> SSN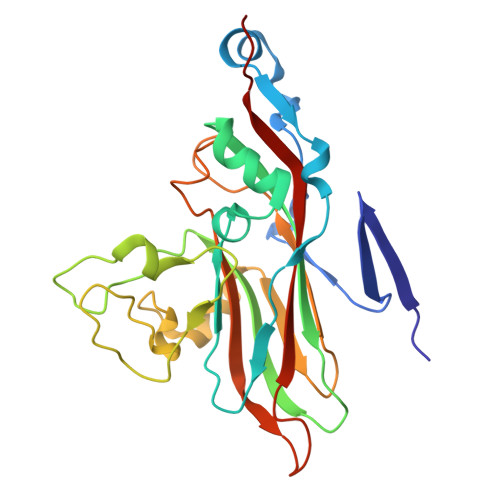VRSITLGNSTITTQESSNVVVGFGVWPSYLSKSKSGSGSTQPTQPDTATERFYTLESVKWQKTDNGWYWKFPDALKDMGLFGQNMLYHFLGRTGWTIHVKCEASRFFQGALLVVCVPQAEKGCAVITRDVNATALDEGDKAKKFTAGSVSSQNGVQTAVYNAAMGVAVGNLTIFPHQWINLKTNNSATIVKPYINSIPMENMYRHFNFTLMVIPFVPLEWSVGACTYVPITVTVAPQNAEYIGLRLA>[6x]C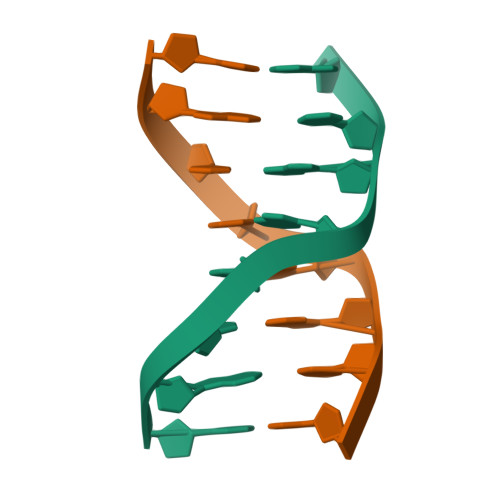GCTAGCG> QYVRIKNWGSGEILHDTL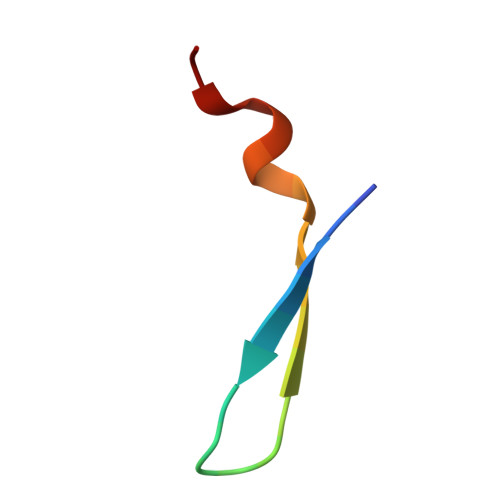HHKATS>[2x]GPPILKELENLSPEEAAHQKAVVETLLQEDPWRVAKMVKSYLQQHNIPQREVVDTTGLNQSHLSQHLNKGTPMKTQKRAALYTWYVRKQREVAQQFTHAGQGGLIEEPTGDELPTKKGRRNRFKWGPASQQILFQAYERQKNPSKEERETLVEECNRAECIQRGVSPSQAQGLGSNLVTEVRVYNWFANRRKEEAFRH

Hepatocyte nuclear factor 1A (HNF-1A) and HNF-4A are transcription factors that engage in crossregulatory gene transcription networks to maintain glucose-stimulated insulin secretion in pancreatic β cells. Variants in the HNF1A and HNF4A genes are associated with maturity-onset diabetes of the young (MODY). HNF-1A and HNF-4A form a crossregulatory loop, in which both factors regulate the respective other’s gene transcription. HNF-1A binds to the P2-HNF4A promoter and activates P2-driven gene transcription.

We therefore recombinantly expressed and purified an HNF-1A construct harboring the DBD (HNF-1A 83-279) and crystallized the DBD:P2 complex using a synthetic P2 oligonucleotide. We refined the crystal structure to 2.3 Å resolution. Two DBD molecules bind to 2 P2 DNA double helices from opposite sides along the helical axis. Both the POUS and the POUH contribute to DNA recognition by HNF-1A. The majority of protein-DNA interactions are mediated by helices α3 and α4 in the POUS, as well as helix α8 in the POUH. Identical measurements with a P2 oligonucleotide revealed a lower affinity (KD = 304 nM ± 134 nM), which was in accordance with our expectations because of the noncanonical HNF-1A binding site in the P2 promoter sequence. A structural alignment of the DBD:RA and DBD:P2 crystal structures revealed a nearly identical conformation of DBD, with an average Cα atom root-mean-square deviation (RMSD) of 0.58 Å. The S.A12>T12 nucleotide change in the P2 promoter sequence leads to a conformational change of the Gln141 side chain, likely due to changes in the base interactions. The polar interactions between the side chains of Gln130 and Gln141 are maintained, but the Gln141 side chain does not interact with the S.T12 base. Arg203 in the P2-bound structure, however, adopts a differently oriented conformation, in which it appears to form a hydrogen bond with the thymine base of S.T14, as well as with AS.A9 and AS.A10 in the complementary strand.> MAVPETRPNHTIYINNLNEKIKKDELKKSLHAIFSRFGQILDILVSRSLKMRGQAFVIFKEVSSATNALRSM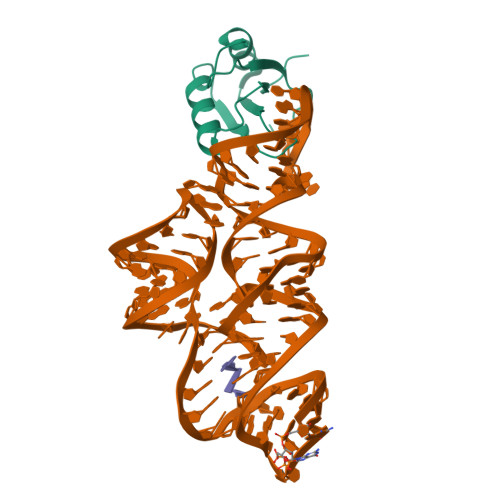QGFPFYDKPMRIQYAKTDSDIIAKMK>[4x]IKKIPMIIGGAERDTSEHEYRELTLNSYKVSIPIINQDDVEAIKSQSVENNLNINQIVNFLYTVGQKWKSENYSRRLTYIRDLVRFLGYSPEMAKLEANWISMILSSKSALYDIVETELGSRHIVDEWLPQGDCYVKAMPKGKSVHLLAGNVPLSGVTSIIRAILTKNECIIKTSSADPFTAIALASSFIDTDEHHPISRSMSVMYWSHNEDIAIPQQIMNCADVVVSWGGYDAIKWATEHTPVNVDILKFGPKKSIAIVDNPVDITASAIGVAHDICFYDQQACFSTQDIYYIGDNIDAFFDELVEQLNLYMDILPKGDQTFDEKASFSLIEKECQFAKYKVEKGDNQSWLLVKSPLGSFGNQPLARSAYIHHVSDISEITPYIENRITQTVTVTPWESSFKYRDVLASHGAERIVESGMNNIFRVGGAHDGMRPLQRLVKYISHERPYTYSTKDVAVKIEQ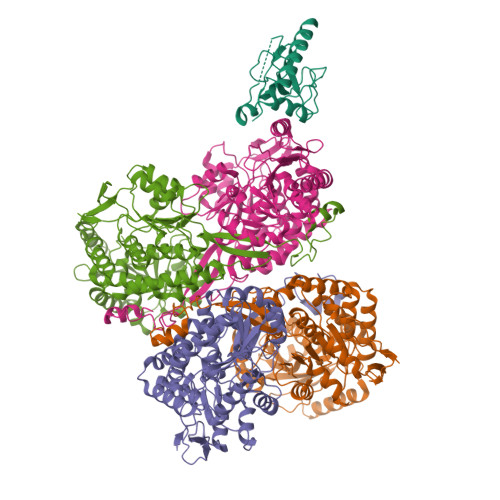TRYLEEDKFLVFVP;> MTITLDICEKDIIVSTEIDDIIFTSSPLDITYDEQERIKHKLILESFRYHYNNNEDYKSFCNTQGVDENISSLDDIPVFPTSMFKYAKICTADESNIENWFTSSGTSGVKSHIARDRVSIERLLGSVNYGMKYLGSFHENQLELVNMGPDRFNAKNVWFKYVMSLVELLYPTTFTVNNDEIDFELTIKSLKEIYNKGKGICLIGPPYFIYLLCQYMKENDIEFNAGNRIFIITGGGWKTKQKQALNRQDFNQLLMETFHLAHESQIRDTFNQVELNTCFFEDNRQRKHVPPWVYARALDPVTLKPVEDGQEGLISYMDASSTSYPTFIVTDDIGIIHTIKAPDPHQGTTIDIVRRLNTREQKGCSLSMSSGLK>GSMASHGNAPPAPVGGAAQTHTQPPVQTAMRIALWNRATHGEQGALQHLLAGLWIQTEISPNSGDIHPLLFFDREHAEITFSRASVQEIFLVDSAHTHRKTVSFLTRNTAISSIRRRLEVTFESHAVIHVRAVEDVARLKIGSTSMWDGQYTRYHAGPASAPSPAAA[9x]

One protein suggested to play a role in T. pallidum dissemination within the host is Tp0751 (also referred to as pallilysin). This protein is a primary target of opsonic antibodies, and thus is predicted to be surface-exposed on T. pallidum, and it binds and degrades host components encountered by T. pallidum during dissemination. The Treponema pallidum protein, Tp0751, possesses adhesive properties and has been previously reported to mediate attachment to the host extracellular matrix components laminin, fibronectin, and fibrinogen. Herein we demonstrate that Tp0751 adopts an eight-stranded beta barrel-containing lipocalin structure, and using a peptide library approach we show that the extracellular matrix component adhesive functionality of Tp0751 is localized to the lipocalin domain.

We also mutated Glu199 to Ala to stabilize the protein for crystallization studies. We next crystallized and determined the three dimensional structure of Tp0751_78A using selenium single wavelength anomalous dispersion (SAD) phasing to a resolution of 2.15 Å. Structural analysis revealed that the C-terminal domain of Tp0751_78A adopts a compact eight-stranded antiparallel beta-barrel with +1 topology, capped by a short 310-like helix and a longer N-terminal helix. The first ordered residue in the Tp0751_78A structure was Gln96 indicating the N-terminal residues Ser78 to Thr95 were either disordered or proteolyzed in the crystal. Analysis clearly revealed an intact N-terminal extension present in the Tp0751_78A crystals indicating that the lack of electron density for the N-terminal residues in the structure reflects disorder and not proteolysis. Comparison of the Tp0751_78A structure against the database of known structures using the DALI server revealed a striking similarity to lipocalin domains, specifically nitrophorins. Ultimately, the classification of Tp0751 as an outlier lipocalin domain, as opposed to a kernel lipocalin, is based on the observation that is does not contain all three SCRs. The SCR1 in Tp0751 localizes to the 310 helix and Strand A, centered on a GxW motif (Gly125 and Trp127 in Tp0751). Although SCR3 is distal in amino acid sequence, residing on Strand H, the key basic residue in this region (Arg226 in Tp0751) stacks on top of the SCR1 Trp and forms a hydrogen bond to the backbone carbonyl of the preceding coil. Although Loop 1 of Tp0751_78A is exposed and partially disordered in the structure, there is no discernable hydrophobic pocket, primarily because Loop 7 caps the hydrophobic core with a stacked Trp-Met pair (right).> MNGTQASNGVLHLDALIIGSGFSGIYLLHKLRDELKLKVKIFEAESDIGGTWNNNRYPGARVDCPVPFYAYSLPEVWQSWNWTELYPNQKEIKSYFDHVDRVLDVRKDCLFHSRVNEGTFDEATGRWTVWTTDGKVATAKYLLVAVGFASKSYLPDWKGLDSFKGTIYHSAHWPEAEEISVKGKKVAVIGTGSTGIQIFQEWAREAEEAFLFQRTPNLCLPMRQQELHAGYQVKDKGEYAD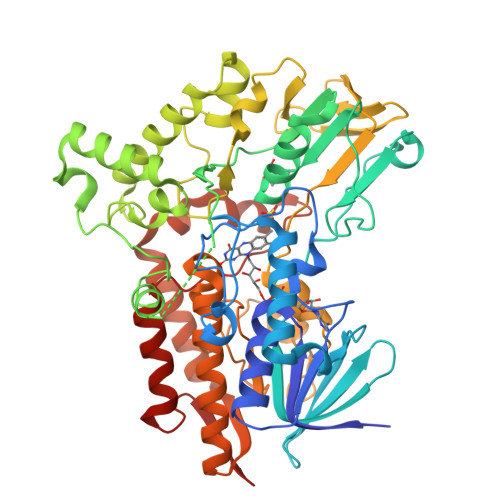YLAECALTFGGLEYQQTPKNTFDASEEEREAFWEDLYQMGGFRFWQNNYQDLLTSLDANREAYNFWARKTRARIQDPKKRDLLAPLEPPYPFGTKRPSLEQDFYEQFNKSNVHIVDTKSQPIVGVTPTGIVTADEKVHEVDIIAVATGFDAVTGGLLRLGLKDVNGVGLDERWKDGMSTYLGMAISGFPNMFLPYSLQAPTAFANGPTLIELQGDWITSLIRKMEMENVQSVTATPHAESAWNDEVNMIANKTLLPLTDSWYMGSNIPGKPVQSLNYLGGLPTYRERCAKVLDEDFFGFAKAHHHHHH>MTKLDKGTVIAAALELLNEVGMDSLTTRKLAERLKVQQPALYWHFQNKRALLDALAEAMLAERHTRSLPEENEDWRVFLKENALSFRTALLSYRDGARIHAGTRPTEPNFGTAETAIRFLCAEGFCPKRAVWALRAVSHYVVGSVL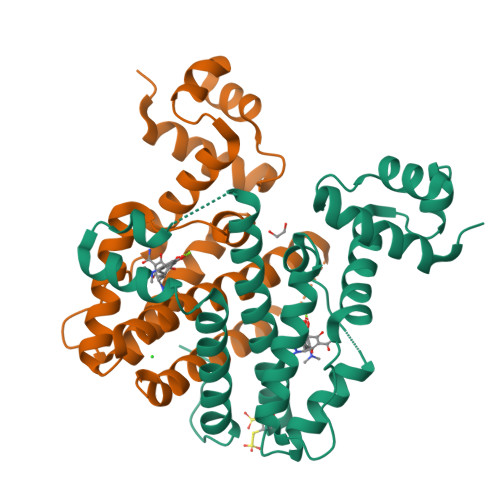EQQASDADERVPDRPDVSEQAPSSFLHDLFHELETDGMDAAFNFGLDSLIAGFERLRSSTTDHHHHHH[4x]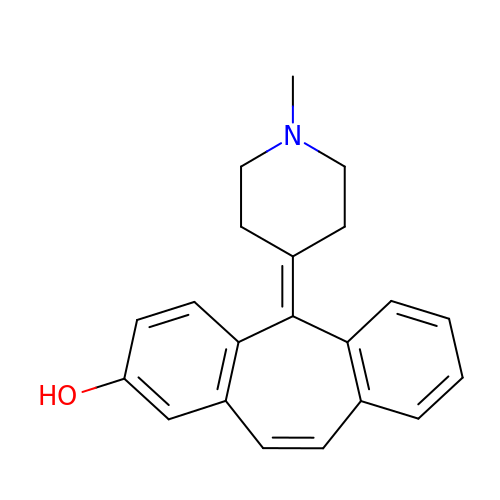2-(1-methylpiperidin-4-ylidene)tricyclo[9.4.0.0^{3,8}]pentadeca-1(11),3(8),4,6,9,12,14-heptaen-6-ol | C21 H21 N O | SJMZFTTXPYYBAG-UHFFFAOYSA-N In recent years, biocatalysis has emerged as a promising recycling methodology for poly­(ethylene terephthalate) (PET), an abundantly produced plastic, due to its potential to selectively depolymerize the polymer under mild conditions. , A number of naturally occurring hydrolase enzymes have been discovered that catalyze the conversion of PET to its constituent monomers, terephthalic acid (TPA) and ethylene glycol (EG). − Most of these PET hydrolases exhibit promiscuous activity related to their native functions as cutinases, lipases, and carboxylesterases. In this study, we use the term ″PET hydrolase″ to denote enzymes with demonstrated PET hydrolytic activity, acknowledging that the observed activity of these enzymes is very likely promiscuous activity. All sequences shared a catalytic domain with the Asp-His-Ser triad within the conserved α/β hydrolase fold, as shown by the alignment of Cα atoms for each Alphafold2 predicted structure against LCC-ICCG using mTm-align. In this study, we applied three consecutive rounds of machine learning and high-throughput (HTP) experimental characterization to discover PET-active hydrolases.

To provide a basis for structural investigations, we selected the most performant enzymes from our Round 1 candidates that also expressed well in the small-scale experiments. Expression of these enzymes was scaled-up, and one enzyme, DP043 from Actinoplanes sp. DH11, was successfully crystallized, with the crystal structure being determined using molecular replacement. While multiple AlphaFold models have been shown to closely correlate with independent crystallographic models of these compact α/β folds, we wanted to validate this here. Alignment of the DP043 AlphaFold3 and crystallographic models shows close alignment, including side chains, with an all-atom RMSD of only 0.266 Å and accurate prediction via Alphafold3 of the location of the Ca2+ ion observed in the crystal structure. The crystal structure revealed a Ca2+ ion, a feature known in other PET hydrolases which has been targeted for rational engineering due to its role in stabilizing the protein. The Ca2+ in the crystal structure of DP043 was not located in the same position as observed in the engineered examples, such as LCC and TfCut2 and further studies would be required to evaluate if the Ca2+ in DP043 serves a similar purpose.

>[2x]AANPYQRGPAPTAASVAAVTGPFATASVSVPRGNGFGGGVIYYPTDTSQGTFGGLAISPGLNGTWPGIAWLGSRLASQGFIVFGIETNNLNDSPTSRGTQLLAALDYLAQRSSVRSRLDPGRLAVAGHSMGGGGALDAALRRPSLKAAIGNAPYLPSNTLAGNRVPTLIYAMQNDTLVPPSRLTSLYNTIPATTERAYLEITGAGHNYIGQPSTTLARTMIPWLKIFIDNDTRFSQFLCPLADQSGIRQYRSSCPLVPATTRALTAAAG CDK16 is a newly recognised member of the CDK protein kinase family that is activated upon binding to the membrane-associated protein cyclin Y (CCNY) or its homologue cyclin Y-like 1 (CCNYL1). The crystal structures of monomeric CDK16 represent the first structures from the PCTAIRE family of CDK kinases. The kinase domain exhibits the classical bilobal architecture intermixed with short insertions that help to define the CDK family fold. The predominantly α-helical C-lobe contains the CDK/MAPK insert, which packs against the αDE and αG helices, as well as a PCTAIRE family specific C-terminal extension that stretches behind the αI helix before folding back to terminate beside the αD helix.

In contrast, the rebastinib complex has a canonical αC helix that includes the PCTAIRE motif, which probably reflects the additional interactions this region forms with the bound inhibitor. The rebastinib co-structure displays an inactive ‘DFG-out, αC-in’ configuration. In this structure, Asp304, Phe305 and Gly306 are flipped into an inverted conformation relative to an active kinase. The activation segment therefore folds antiparallel to the β1 strand and occludes the front of the ATP pocket. As anticipated, the binding of rebastinib is facilitated by an inverted conformation of the ‘DFG motif’, which creates an extra pocket for inhibitor binding below the αC helix. Rebastinib forms a total of five hydrogen bonds with the ATP-binding pocket of CDK16, as similarly observed in the equivalent ABL structure. The carboxamide-substituted pyridine ring forms two hydrogen bonds with the backbone amide and carbonyl of the ATP-hinge residue, Leu243. The urea moiety's nitrogens also form two hydrogen bonds with Glu211 from the αC ‘PCTAIRE’ motif. The central phenyl ring is sandwiched between the gatekeeper residue Phe240 and the flipped-out Phe305 (DFG motif), providing strong π–π packing interactions.

>METYIKLDKLGEGTYATVYKGKSKLTDNLVALKEIRLEHEEGAPCTAIREVSLLKDLKHANIVTLHDIIHTEKSLTLVFEYLDKDLKQYLDDCGNIINMHNVKLFLFQLLRGLAYCHRQKVLHRDLKPQNLLINERGELKLADFGLARAKSIPTKTYDNEVVTLWYRPPDILLGSTDYSTQIDMWGVGCIFYEMATGRPLFPGSTVEEQLHFIFRILGTPTEETWPGILSNEEFKTYNYPKYRAEALLSHAPRLDSDGADLLTKLLQFEGRNRISAEDAMKHPFFLSLGERIHKLPDTTSIFALKEIQLQKEASLRSAHHHHHH[2x]>[2x]MWDVIVVG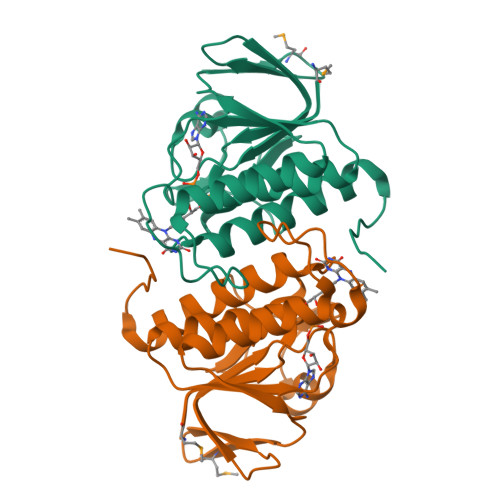GGPSGLSAALFLARAGLKVLVLDGGRSKVKGVSRVPNYPGLLDEPSGEELLRRLEAHARRYGAEVRPGVVKGVRDMGGVFEVETEEGVEKAERLLLCTHKDPTLPSLLGLTRRGAYIDTDEGGRTSYPRVYAAGVARGKVPGHAIISAGDGAYVAVHLVSDLRGEPYKDHAL>[6x]SMPPHGELQYLGQIQHILRCGVRKDDRTGTGTLSVFGMQARYSLRDEFPLLTTKRVFWKGVLEELLWFIKGSTNAKELSSKGVKIWDANGSRDFLDSLGFSTREEGDLGPVYGFQWRHFG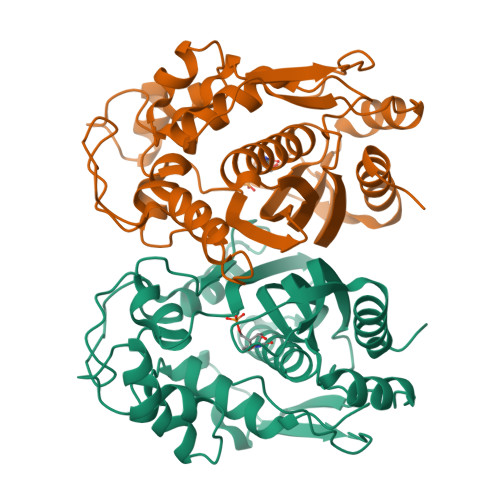AEYRDMESDYSGQGVDQLQRVIDTIKTNPDDRRIIMCAWNPRDLPLMALPPCHALCQFYVVNSELSCQLYQRSGDMGLGVPFNIASYALLTYMIAHITGLKPGDFIHTLGDAHIYLNHIEPLKIQLQREPRPFPKLRILRKVEKIDDFKAEDFQIEGYNPHPTIKMEMAV> MAFHE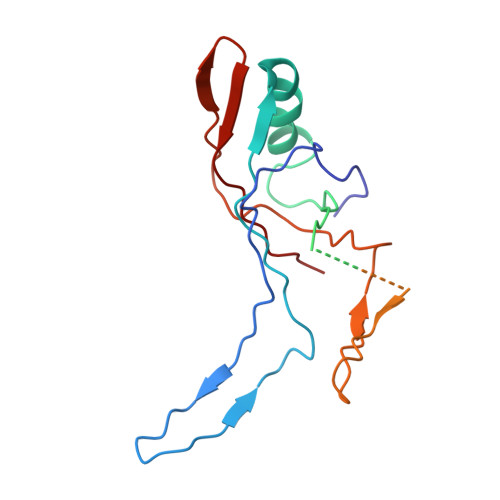VRFPANLSFGSVGGPERRTEIVTLSSGHEERNSPWAHSRRHYDAGVGLRSLDDVERLIAFFEARGGQLHGFRWKDWADFKSCPASRAVAHEDQLIGMGDGVTTAFQLVKTYVSGGQSYLRPIVKPVEGTVKLGIAGDHQAEAVNFAVDHATGIVSFNEPPPQGARVTAGFEFDVPVRFDTDRIAVSVQSFQAGDLPQVPVVEVRI> RVADTVGTGPTNSEAIPALTAAETGHTSQVVPGDTMQTRHVKNYHSRSESTIENFLCRSACVYFTEYENSGAKRYAEWVLTPRQAAQLRRKLEFFTYVRFDLELTFVITSTQQPSTTQNQDAQILTHQIMYVPPGGPVPDKVDSYVWQTSTNPSVFWTEGNAPPRMSIPFLSIGNAYSNFYDGWSEFSRNGVYGINTLNNMGTLYARHVNAGSTGPIKSTIRIYFKPKHVKAWI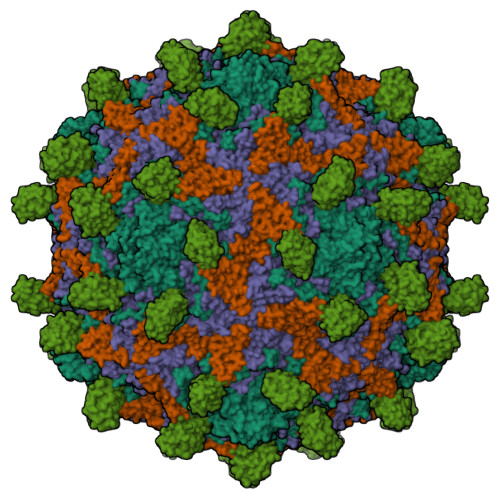PRPPRLCQYEKAKNVNFQPSGVTTTRQSITTMT;> SPTVEECGYSDRARSITLGNSTITTQECANVVVGYGVWPDYLKDSEATAEDQPTQPDVATCRFYTLDSVQWQKTSPGWWWKLPDALSNLGLFGQNMQYHYLGRTGYTVHVQCNASKFHQGCLLVVCVPEAEMGCATLDNTPSSAELLGGDSAKEFADKPVASGSNKLVQRVVYNAGMGVGVGNLTIFPHQWINLRTNNSATIVMPYTNSVPMDNMFRHNNVTLMVIPFVPLDYCPGSTTYVPITVTIAPMCAEYNGLRLAGHQ;> GLPTMNTPGSCQFLTSDDFQSPSAMPQYDVTPEMRIPGEVKNLMEIAEVDSVVPVQNVGEKVNSMEAYQIPVRSNEGSGTQVFGFPLQPGYSSVFSRTLLGEILNYYTHWSGSIKLTFMFCGSAMATGKFLLAYSPPGAGAPTKRVDAMLGTHVVWDVGLQSSCVLCIPWISQTHYRYVTSDEYTAGGFITCWYQTNIVVPADAQSSCYIMCFVSACNDFSVRLLKDTPFISQQNFFQ;> MGAQVSTQKTGAHETGLNASGNSIIHYTNINYYKDAASNSANRQDFTQDPGKFTEPVKDIMIKSLPALN;> MSITTPEEMIEKAKGETAYLPCKFTLSPEDQGPLDIEWLISPADNQKVDQVIILYSGDKIYDDYYPDLKGRVHFTSNDLKSGDASINVTNLQLSDIGTYQCKVKKAPGVANKKIHLVVLVKPSGARCYVDGSEEIGSDFKIKCEPKEGSLPLQYEWQKLSDSQKMPTSWLAEMTSSVISVKNASSEYSGTYSCTVRNRVGSDQCLLRLNVVPPSNKALEHHHHHH2-({5-bromo-2-[(3,4,5-trimethoxyphenyl)amino]pyrimidin-4-yl}oxy)-N-methylbenzene-1-carboximidic acid | C21 H21 Br N4 O5 | 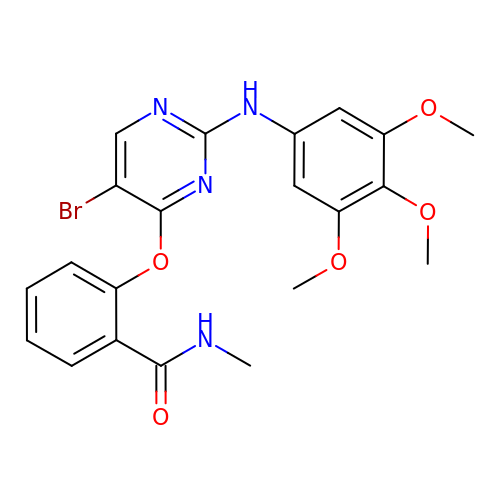NEXGBSJERNQRSV-UHFFFAOYSA-N> MTDTASKYAVKLKTNFEDPKWVNRHKFMFNFLDINGNGKI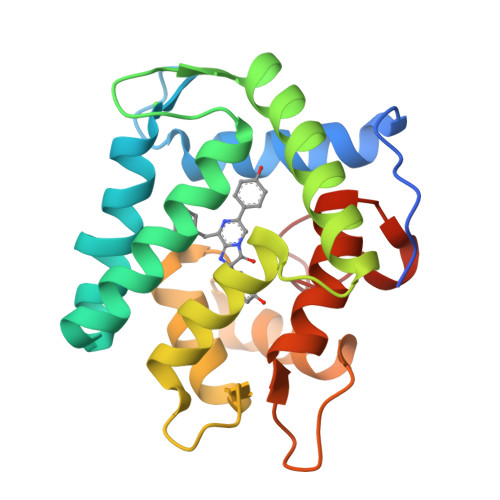TLDEIVSKASDDICAKLGATPAQTQRHQEAVEAFFKKIGLDYGKEVEFPAFVNGWKELAKHDLKLWSQNKKSLIRNWGEAVFDIFDKDGSGSISLDEWKTYGGISGICPSDEDAEKTFKHCDLDNSGKLDVDEMTRQHLGFWYTLDPNADGLYGNFVP> MVQELSIERLLEMESLVADPSEEFQFLRVGPDSNVPPKFRAPVSSLCQIGNKQIAALVVWARDIPHFSQLEMEDQILLIKGSWNELLLFAIAWRSMEFLTEERDGVDGTGNRTTSPPQLMCLMPGMTLHRNSALQAGVGQIFDRVLSELSLKMRTLRVDQAEYVA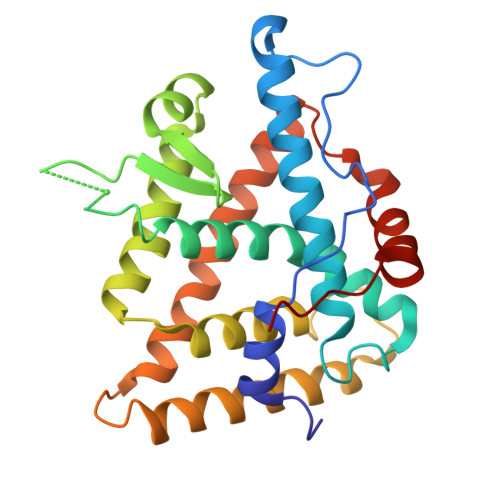LKAIILLNPDVKGLKNRQEVEVLREKMFLCLDEYCRRSRSSEEGRFAALLLRLPALRSISLKSFEHLFFFHLVADTSIAGYIRDALRNHAPPIDTNMM> MTIIIASDNAIIEINQALNTILSQYLNITGQNIDIRFDLPEINSIQSEPTVSVFLYEIHEDLQLRSAESRRYNPSTNTL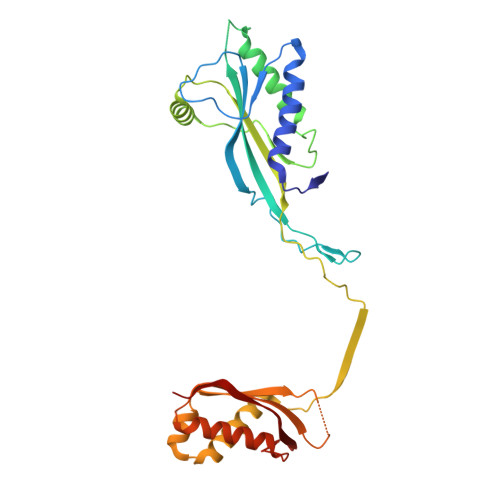LPGWVNINCNYLITYWDASKPSSDSSSPDSQPNNQAAQVMTRILNALINNRQLTGLPGAYTRIIPQQENLNSLGNFWQALGNRPRLSLLYSITVPMKLKNIEDNVIPVSKISASVDQKPNLDNSQINQALIDKLCVELGGTEDVRLALAKVNLTTKPDTENNQNQENESVIVEVSGITSVTYLPQIKDTLTKWKSSQEAIVKINGVSIVVSKENADKLIGI>GSPCPGACVCYNEPKVTTSCPQQGLQAVPTGIPASSQRIFLHGNRISHVPAASFQSCRNLTILWLHSNALARIDAAAFTGLTLLEQLDLSDNAQLHVVDPTTFHGLGHLHTLHLDRCGLRELGPGLFRGLAALQYLYLQDNNLQALPDNTFRDLGNLTHLFLHGNRIPSVPEHAFRGLHSLDRLLLHQNHVARVHPHAFRDLGRLMTLYLFANNLSMLPAEVLMPLRSLQYLRLNDNPWVCDCRARPLWAWLQKFRGSSSEVPCNLPQRLADRDLKRLAASDLEGCAVASGPFRPIQTSQLTDEELLSLPKCCQPDAA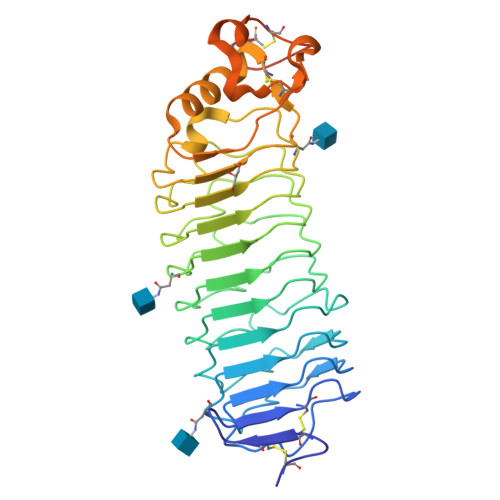DKASVLEAAAHHHHHH[2x]> GSPNSRVDELGFNEAERQKILDSNSSLMRNANEVRDKFIQNYATSLKDSNDPQDFLRRVQELRINMQKNFISFDAYYNYLNNLVLASYNRCKQEKTFAESTIKNELTLGEFVAEISDN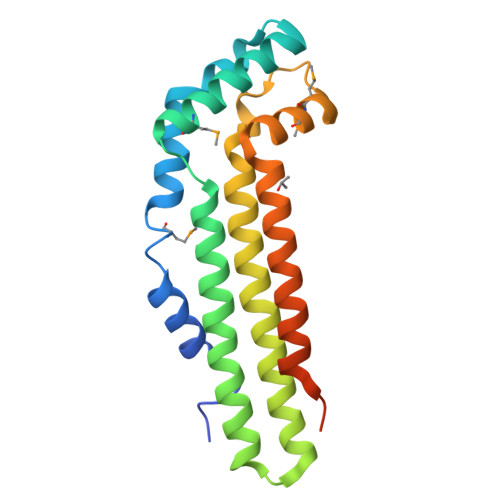FNNFTCDEVARISDLVASYLPREYLPPFIDGNMMGVAFQILGIDDFGKKLNEIVQDIGTKYIILSKNKTYLTSLERAKLITQLKLNLE>[15x]GDEMVTRVVPVRNVSVRELAPLLRQLNDNAGGGNVVHYDPSNVLLITGRAAVVNRLVEVVRRVDKAGDQEVDIIKLKYASAGEMVRLVTNLNKDGNSQGGNTSLLLAPKVVADERTNSVVVSGEPKARARIIQMVRQLDRELQSQGNTRVFYLKYGKAKDMVEVLKGVSSSIEADKKGGGTATTAGGGASIGGGKLAISADETTNALVITAQPDVMAELEQVVAKLDIRRAQVLVEAIIVEIADGDGLNLGVQWANTNGGGTQFTNAGPGIGSVAIAAKDYKDNGTTTGLAKLAENFNGMAAGFYQGNWAMLVTALSTNTKSDILSTPSIVTMDNKEASFNVGQEVPVQTGTQNSTSGDTTFSTIERKTVGTKLVLTPQINEGDSVLLTIEQEVSSVGKQATGTDGLGPTFDTRTVKNAVLVKSGETVVLGGLMDEQTKEEVSKVPLLGDIPVLGYLFRSTSNNTSKRNLMVFIRPTILRDANVYSGISSNKYTLFRAQQLDAVAQEGYATSPDRQVLPEYGQD

Pathogenic bacteria commonly employ the Type II Secretion System (T2SS) for the release of protein toxins. The system includes an inner membrane platform of GspC-E-F-L-M, a periplasmic pseudopilus composed of GspG-H-I-J-K and the outer membrane secretion channel GspD, called the secretin. In numerous species the targeting, assembly and stability of the T2SS secretin in the outer membrane require the function of a small lipoprotein that binds to its C-terminal region (the S-domain) and serves to pilot secretin monomers from the inner to the outer membrane via the LOL lipoprotein sorting pathway. In this study we used cryo-electron microscopy to characterize the structure of the secretins from V. vulnificus and A. hydrophila and in addition determined the crystal structure of EpsS from V. vulnificus.

First, we determined the cryo-EM structure of A. hydrophila ExeD as the paradigm of a secretin that is assembled through the actions of the ExeAB accessory complex. Analyses of top views of class averages revealed that, for both secretins, symmetry is unambiguously pentadecameric (C15 symmetry). The resolutions of the resulting symmetrized maps were estimated to be in the range of 3.4 Å for EpsD and 3.7 Å for ExeD by employing the gold standard FSC criterion. In ExeD, the sequence corresponding to the β-hairpin is absent and the structure is finalized by the β-lip, a common feature seen in both structures. The inner membrane ExeAB complex is both necessary and sufficient for the assembly of ExeD; in accordance with this, the Aeromonads do not have known pilotins. However, sequence comparisons reveal that ExeD does contain a recognizable S-domain including residues that could potentially correspond to helix α-12, a fully solvent-exposed, 8-residue helix that has been reported to bind pilotins in analogous regions in other secretins. In our ExeD sequence, for example, the conserved Ala-Phe motif is absent and is replaced by Lys-Gln, residues whose high polarity would not be able to play the same roles of the two hydrophobic amino acids of the motif. In addition, in our cryo-EM structure of ExeD, the last visible residue in the electron density map is Asp620. This indicates that the C-terminal tail, which includes the region discussed above, is flexible and not traceable and most probably does not fold into a stable domain. In contrast, however, the ExeD-EpsD-S variant, in which the EpsD α11 helix-containing region was also exchanged into ExeD, was both assembled in lower amounts and significantly compromised in function once assembled, suggesting that the interactions between this helix and the neighbouring monomer that are evident in the cryo-EM structure play an important role in both the assembly and the function of the secretin.>MQKQRTTSQWRELDAAHHLHPFTDTASLNQAGARVMTRGEGVYLWDSEGNKIIDGMAGLWCVNVGYGRKDFAEAARRQMEELPFYNTFFKTTHPAVVELSSLLAEVTPAGFDRVFYTNSGSESVDTMIRMVRRYWDVQGKPEKKTLIGRWNGYHGSTIGGASLGGMKYMHEQGDLPIPGMAHIEQPWWYKHGKDMTPDEFGVVAARWLEEKILEIGADKVAAFVGEP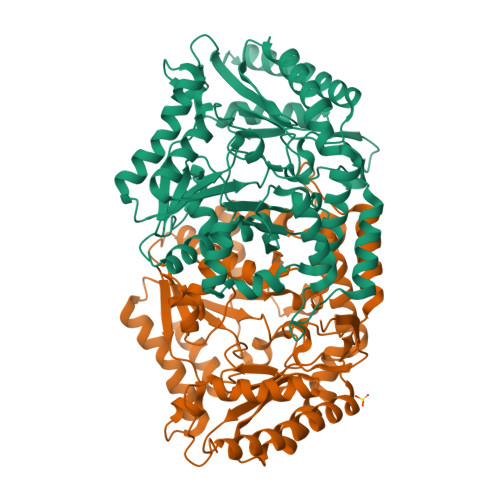IQGAGGVIVPPATYWPEIERICRKYDVLLVADEVICGFGRTGEWFGHQHFGFQPDLFTAAKGLSSGYLPIGAVFVGKRVAEGLIAGGDFNHGFTYSGHPVCAAVAHANVAALRDEGIVQRVKDDIGPYMQKRWRETFSRFEHVDDVRGVGMVQAFTLVKNKAKRELFPDFGEIGTLCRDIFFRNNLIMRACGDHIVSAPPLVMTRAEVDEMLAVAERCLEEFEQTLKARGLA[2x]>MRVAFSAARTSNLAPGTLDQPIVFDLLLNNLGETFDLQLGRFNCPVNGTYVFIFHMLKLAVNVPLYVNLMKNEEVLVSAYANDGAPDHETASNHAILQLFQGDQIWLRLHRGAIYGSSWKYSTFSGYLLYQDLEH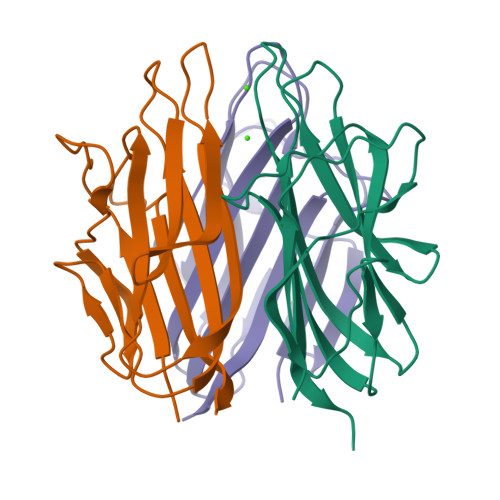HHHHH[6x]>[2x]MWVKILSVVGARPQFIKAAAVSRVLRASPGVREVLVHTGQHYDDNMSQVFFEELEIPDPDYHLGIGGGTHGQNTGRMLEAIEGVLLKEKPDWVLVYGNTDSTLAGALAAVKLHIPVAHVEAGLRSFNRRMPEEINRILTDHASDLLFAPTETAVQNLLREGIPENRIHLVGDVMYDAALHYGAKAERKSRILERLGLQAKGYVLATIHRAENTDDQERLRVILEALAEVHQEVPVVFPVHPRTRKRAEAFGLGSYLEKVVALEPVGYLDMVMLEKNARLIVTDSGGVQKEAYFYRVPCVTVREETEWVELLKAEWNYLAAPQNAKDLALTILHRMRTKGVEIDLYGDGRASQKISDFLRKVGIRTLEHHHHHH

The final step in the pathway is catalyzed by a 2-epimerase, which utilizes UDP-2,3-diacetamido-2,3-dideoxy-d-glucuronic acid as its substrate. The focus of this investigation is on the ORF WP_011172736, which we demonstrate encodes for a 2-epimerase. We have also demonstrated that the T. thermophilus enzyme is allosterically regulated by UDP-GlcNAc. Whereas the sugar 2-epimerases that function on UDP-GlcNAc have been the focus of past biochemical and structural analyses, this is the first detailed investigation of a 2-epimerase that specifically utilizes UDP-2,3-diacetamido-2,3-dideoxy-d-glucuronic acid as its substrate.

In an attempt to trap the UDP-sugar substrate in the active site, we subsequently constructed the D98N variant and crystallized it at pH 7.0 in the presence of UDP-GlcNAc3NAcA (structure 4). Again, the asymmetric unit contained a dimer (α-carbons of the two subunits superimpose with an RMSD of 0.4 Å). The model was refined to an overall R-factor of 19.5% at 2.2 Å resolution. Unambiguous electron density corresponding to the UDP-substrate was observed in each subunit. Surprisingly, however, in subunits A and B, there were also electron densities corresponding to UDP and UDP-GlcNAc, respectively, albeit at lower occupancies as can be seen in Figure 7, A and B. Importantly, these ligands were not included in the crystallization trials. The UDP in subunit A and the UDP-GlcNAc in subunit B align closely with the exception of their β-phosphoryl groups. In subunit A, the β-phosphoryl group does not lie within 3.2 Å of any protein atoms, whereas in subunit B, it forms an electrostatic interaction with Arg 242. Although the electron densities of the exogenous ligands in structure 4 were unambiguous, we utilized a combination of protein denaturation, HPLC, and mass spectrometry to verify their presence in the purified protein before the crystallization trials. As described in Experimental procedures, they were identified as UDP-GlcNAc and UDP. When the denaturation protocol was performed with the WT enzyme, the same two compounds were observed, but at only a couple of percent the abundance of that observed for the D98N variant as shown in Figure 10.>MENIKKMGF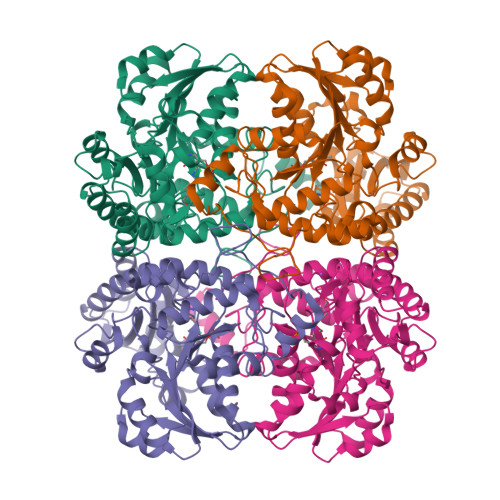ATKAIHGGHIGDKQFGSLATPIYQTSTFIFDSAEQGGRRFAGEESGYIYSRLGNPTSTEVENKLALLEGGEAAVVAASGMGAIAASLWSALKSGDHVVASDTLYGCTFALLNHGLTRYGVEVTFVDVSNLDEVKNALKPNTKVVYLETPANPTLKVTDIRKISNMVHESNKECFVFVDNTFCTPYIQRPLELGADVVVHSATKYLNGHGDVIAGFAVGKEEFINQVKLFGIKDMTGSVTGPFESFLIIRGMKTLQLRMEKHCKNAMEVAKFLESHPAVEKVYYPGLESFKYYQLAREQMKLPGAMISFELKGGVEEGKIVMNNVKLATLAVSLGDSETLIQHPASMTHSPYTAEERKAAGISDGLVRLSVGLEDAEDIIDDLKQALDLIVK[2x]> TIEKRYDFVFLFDVQDG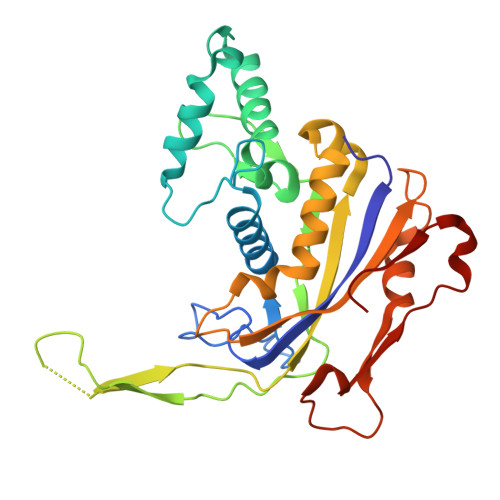NPNGDPDAGNLPRIDPQTGEGLVTDVCLKRKVRNFIQMTQNDEHHDIFIREKGILNNLIDEAHEQENVKGKEKGEKTEAARQYMCSRYYDIRTFGAVMTTGKNAGQVRGPVQLTFSRSIDPIMTLEHSITRMAVTNEKDASETGDNRTMGRKFTVPYGLYRCHGFISTHFAKQTGFSENDLELFWQALVNMFDHDHSAARGQMNARGLYVFEHSNNLGDAPADSLFKRIQVVKKDGVEVVRSFDDYLVSVDDKNLEETKLLRKLGG>NLDQMKKDFIANVSHELRTPISLLQGYTESIVDGIVTEPDEIKESLAIVLDESKRLNRLVNELLNVARMDAEGLSVNKEVQPIAALLDKMKIKYRQQADDLGLNMTFNYCKKRVWSYDMDRMDQVLTNLIDNASRYTKPGDEIAITCDENESEDILYIKDTGTGIAPEHLQQVFDRFYKVDAARTRGKQGTGL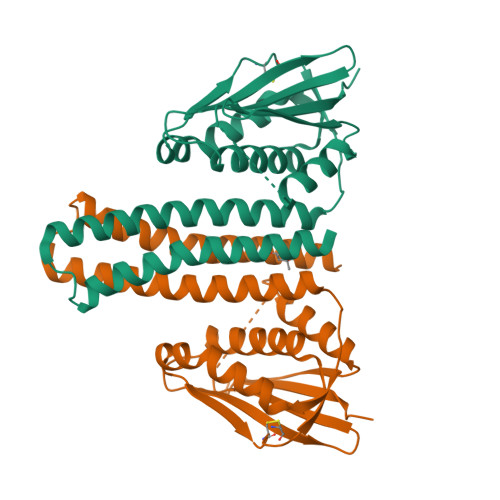GLFICKMIIEEHGGSIDVKSELGKGTTFIIKLPKPE[2x]>MSLEAVTILLADDEAILLLDFESTLTDAGFLVTAVSSGAKAIEMLKSGAAIDGVVTDIRFCQPPDGWQVARVAREIDPNMPIVYISGHAALEWASNGVPDSIILEKPFTSAQLITAVSQLLNAREGH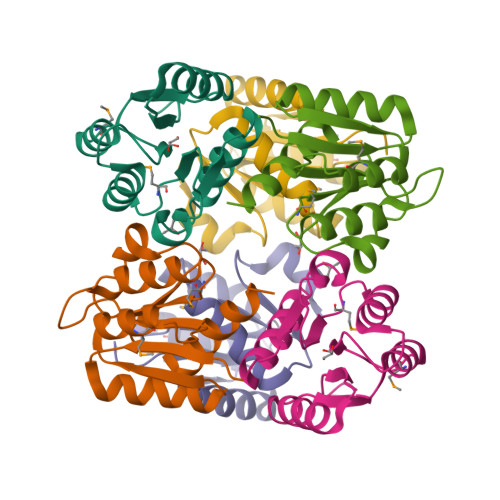HHHHH[3x]> SDAHDEETFEEFTARYEKEFDEAYDLFEVQRVLNNCFSYDLVPAPAVIEKALRAARRVN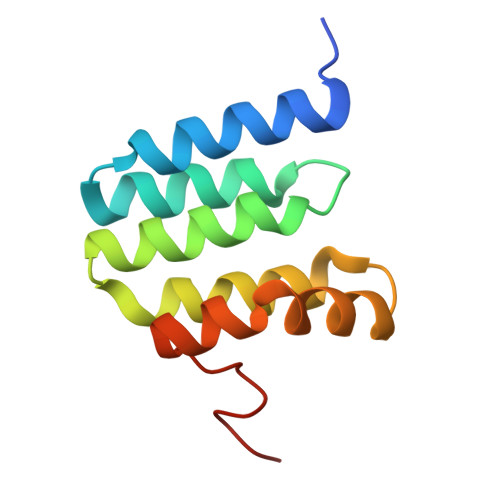DLPTAIRVFEALKYKVENEDQYKAYLDELKDVRQELGVPLKEELFPSSS> EPCVEVVPNITYQCMELNFYKIPDNLPFSTKNLDLSFNPLRHLGSYSFFSFPELQVLDLSRCEIQTIEDGAYQSLSHLSTLILTGNPIQSLALGAFSGLSSLQKLVAVETNLASLENFPIGHLKTLKELNVAHNLIQSFKLPEYFSNLTNLEHLDLSSNKIQSIYCTDLRVLHQMPLLNLSLDLSLNPMNFIQPGAFKEIRLHKLTLRNN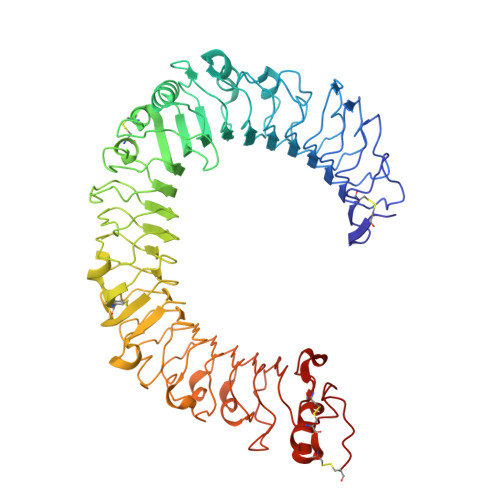FDSLNVMKTCIQGLAGLEVHRLVLGEFRNEGNLEKFDKSALEGLCNLTIEEFRLAYLDYYLDDIIDLFNCLTNVSSFSLVSVTIERVKDFSYNFGWQHLELVNCKFGQFPTLKLKSLKRLTFTSNKGGNAFSEVDLPSLEFLDLSRNGLSFKGCCSQSDFGTTSLKYLDLSFNGVITMSSNFLGLEQLEHLDFQHSNLKQMSEFSVFLSLRNLIYLDISHTHTRVAFNGIFNGLSSLEVLKMAGNSFQENFLPDIFTELRNLTFLDLSQCQLEQLSPTAFNSLSSLQVLNMSHNNFFSLDTFPYKCLNSLQVLDYSLNHIMTSKKQELQHFPSSLAFLNLTQNDFACTCEHQSFLQWIKDQRQLLVEVERMECATPSDKQGMPVLSLNITCQMNK> SNANTPQEAQQVDMWKKYIQWEKSNPLRTEDQTLITKRVMFAYEQCLLVLGHHPDIWYEAAQYLEQSSKLLAEKGDMNNAKLFSDEAANIYERAISTLLKKNMLLYFAYADYEESRMKYEKVHSIYNRLLAIEDI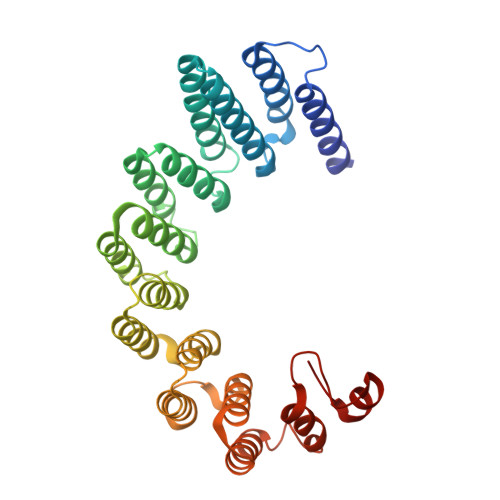DPTLVYIQYMKFARRAEGIKSGRMIFKKAREDTRTRHHVYVTAALMEYYCSKDKSVAFKIFELGLKKYGDIPEYVLAYIDYLSHLNEDNNTRVLFERVLTSGSLPPEKSGEIWARFLAFESNIGDLASILKVEKRRFTAFKEEYEGKETALLVDRYKFMDLYPCSASELKALGYKDV>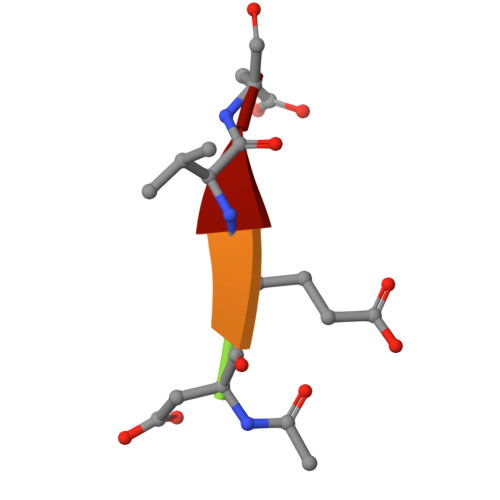 XDEVD>GIDPFTDREKQQLSIEAARLYYQSDYSQQQIAEQLNISRPTVSRLLQYAKEKGYVQIRVMDPFEDLDALGSILEEKYGLLEAHVVFSPTPDYAGITHDLSRYGAEYMHETVKDGDIVGVSWGTTMYQIAQNMQPKQVKGVEVVQLKGGISHSRVNTYSAETIQLFAEAFQTMPRYLPLPVVFDNADVKRMVEKDRHIERIIEMGKQANIALFTVGTVRDEALLFRLGYFNEEEKALLKKQAVGDICSRFFDAKGNICSSAINDRTIGVELQDLRLKERSIL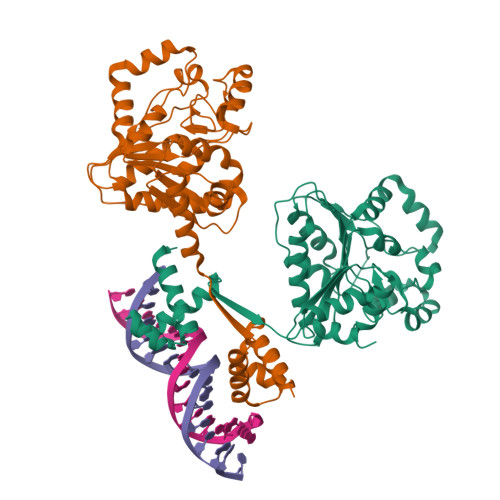VAGGSRKVSSIHGALTGKYANVLIIDQHTARALVNDL[4x]> SMGKKSRVKTQKSGTGATATVSPKEILNLTSELLQKCSSPAPGPGKEWEEYVQIRTLVEKIRKKQKGLSVTFDGKREDYFPDLMKWASENGASVEGFEMVNFKEEGFGLRATRDIKAEE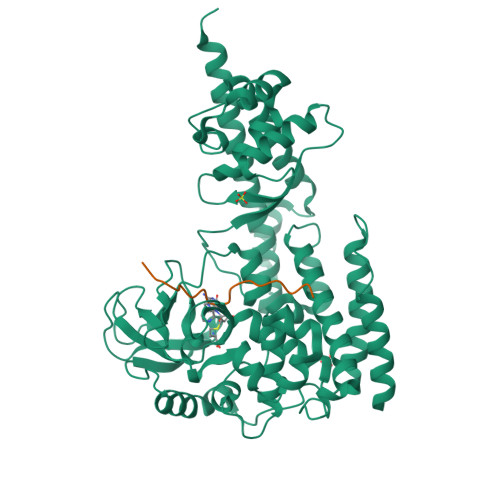LFLWVPRKLLMTVESAKNSVLGPLYSQDRILQAMGNIALAFHLLCERASPNSFWQPYIQTLPSEYDTPLYFEEDEVRYLQSTQAIHDVFSQYKNTARQYAYFYKVIQTHPHANKLPLKDSFTYEDYRWAVSSVMTRQNQIPTEDGSRVTLALIPLWDMCNHTNGLITTGYNLEDDRCECVALQDFRAGEQIYIFYGTRSNAEFVIHSGFFFDNNSHDRVKIKLGVSKSDRLYAMKAEVLARAGIPTSSVFALHFTEPPISAQLLAFLRVFCMTEEELKEHLLGDSAIDRIFTLGNSEFPVSWDNEVKLWTFLEDRASLLLKTYKTTIEEDKSVLKNHDLSVRAKMAIKLRLGEKEILEKAVKSAAVNREYYRQQMEEKAP;> TLKYPIEXGIVTNWDD> MHHHHHHSSGRENLYFQGPPARVRVAVRLRPFVDGTAGASDPPCVRGMDSCSLEIANWRNHQETLKYQFDAFYGERSTQQDIYAGSVQPILRHLLEGQNASVLAYGPTGAGKTHTMLGSPEQPGVIPRALMDLLQLTREEGAEGRPWALSVTMSYLEIYQEKVLDLLDPASGDLVIREDCRGNILIPGLSQKPISSFADFERHFLPASRNRTVGATRLNQRSSRSHAVLLVKVDQRERLAPFRQREGKLYLIDLAGSEDNRRTGNKGLRLKESGAINTSLFVLGKVVDALNQGLPRVPYRDSKLTRLLQDSLGGSAHSILIANIAPERRFYLDTVSALNFAARSKEVINRPFTNE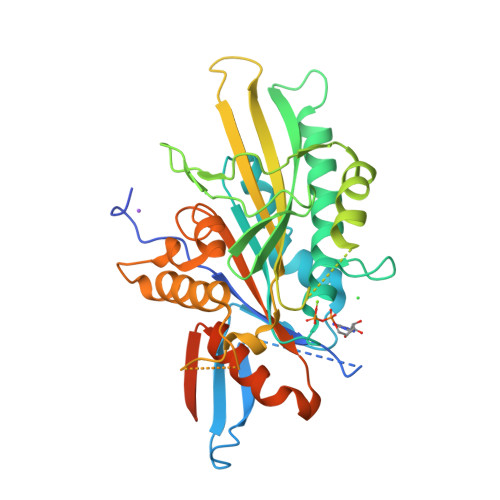SLQPHALGPVKLSQKELLGPPEAK>[3x]GSHMTTDAPSFNLITQPWLPVQYRDGTEKELSLLEVFKQAPLLRRLVGDVPTQEFALLRLLLAILHDAIGGPEDSDEWAELWTQDEAEQQLPFDCIASYLEQYYHRFDLLHPTTPFFQVADLHTQKNDV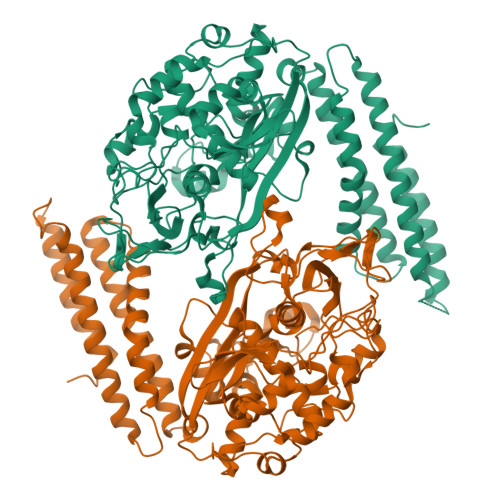FSLDRIVADVPNGELFFTMRARGVDRLSFAEAARWLVHAHAYDTSGIKSGAVGDPRAKGGKGYPQGVSWAGNLGGILVEGANLYETLLLNLVAFDTDNLIVTPEDRPAWRQPPTTAAPADDEELAQRPYGLCDLYTWQSRRIRLHYDADGVYGVLLAYGDPLAPHNKHNHEPMTAWRRSPAQEKKLKKPQVYLPREHDPTRSAWRGLGALVAGEASGAEQRGEAAAIVRPRILDWVARLVNEGFLPEDYFIRTRLIGVSYGTQQAVIDEIVDDHVAMAVVLLHERDSGLGRTAIKAVEDAEKAVTVLGGLAADLAKAAGADPETPRAAARDRGFGMLDGPFRTWLATLAPGTDATERRRAWQQKAHRIISDLGRQLVAEAGEAAWNGRVIKGKNTDVWLNASRADLKFRAELKKELPMATSEQTGEAAS> GRPRTTXF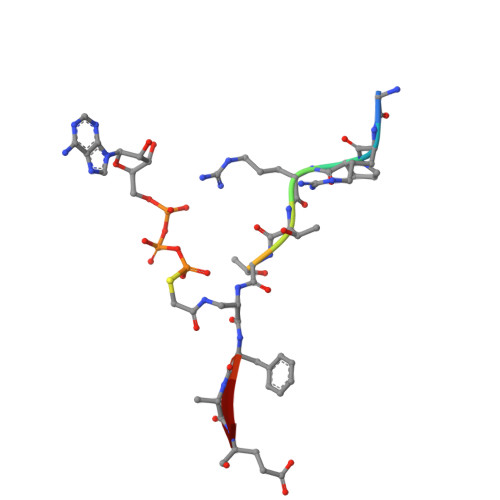AE>AEHHHHHHLVPRGSIAIDDSAAVQRLTGLLNKAQTLTARFSQLTLDGSGTRLQETAGQLSLKRPGLFRWHTDAPNEQLLISNGEKVWLYDPDLEQVTIQKLDQRLTQTPALLLSGDISKISESFAITYKEGGNVVDFVLKPKTKDTLFDTLRLSFRS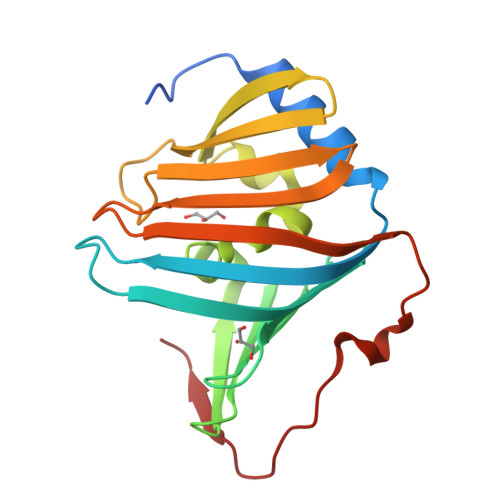GKVNDMQMIDGVGQRTNILFFDVKMNEALDAKQFTFDVPPGVDVIQE[2x]Proteins of the dynamin superfamily mediate membrane fission, fusion, and restructuring events by polymerizing upon lipid bilayers and forcing regions of high curvature. The family consists of the classical dynamins and the dynamin-like proteins (DLPs). They group through common sequence organization and minimally contain an N-terminal GTPase domain, a middle domain, and a C-terminal GTPase effector domain (GED). Other than GBP1, an exception comes from the full-length crystal structure of a bacterial dynamin-like protein (BDLP) from the cyanobacterium Nostoc punctiforme. The BDLP GTPase domain dimerizes and forms the tube surface, the GTPase effector domain (GED) mediates self-assembly, and the paddle region contacts the lipids and promotes curvature.

In this work, we show the electron cryomicroscopy reconstruction of a bacterial dynamin-like protein (BDLP) helical filament decorating a lipid tube at ∼11 Å resolution. We fitted the BDLP crystal structure and produced a molecular model for the entire filament. The BDLP tube reconstruction reveals a tightly packed helical surface coating (50 nm diameter) dominated by dimeric globular densities that represent the asymmetric unit, and that connect as a zigzag with a vertical rise of 64.4 Å (correlates to Bessel order, n = −11). With the SAM label used as an anchor, the BDLP trunk was fitted into a radial spoke with the paddle oriented toward the membrane. However, the density preferentially fits the closer dimer observed in the dynamin-related human GBP1 GTPase domain with bound GDP-AlF3 (Ghosh et al., 2006). With the GTPase domain, neck and trunk docked, application of the helical parameters (rise = 3.1926 Å, rotation = 63.815°) to the asymmetric unit generates a fitted model of the complete helical filament. Nucleotide and lipid binding drive an intramolecular rearrangement in which the BDLP neck rotates ∼135° around proposed hinges 1a and 1b away from the trunk. The GTPase domain also turns ∼70° around two hinge regions so that the nucleotide binding pocket no longer points out along the trunk-neck axis but rests orthogonal to the axis. Analysis of two neighboring BDLP dimers shows that both the helical middle domain and GED run the full length of the extended molecule, making intimate contact with each other and, importantly, through a two-fold symmetry axis, making extensive contact in the neighboring molecule with their equivalent. The BDLP trunk tips just touch the outside of the inner lipid ring and form densely packed (left-handed 11-start) helices that push apart the phospholipid heads of the outer leaflet and restrict them to the spacing between each turn (∼50% of the volume in this region).

>MVNQVATDRFIQDLERVAQVRSEMSVCLNKLAETINKAELAGDSSSGKLSLERDIEDITIASKNLQQGVFRLLVLGDMKRGKSTFLNALIGENLLPSDVNPCTAVLTVLRYGPEKKVTIHFNDGKSPQQLDFQNFKYKYTIDPAEAKKLEQEKKQAFPDVDYAVVEYPLTLLQKGIEIVDSPGLNDTEARNELSLGYVNNCHAILFVMRASQPCTLGERRYLENYIKGRGLTVFFLVNAWDQVRESLIDPDDVEELQASENRLRQVFNANLAEYCTVEGQNIYDERVFELSSIQALRRRLKNPQADLDGTGFPKFMDSLNTFLTRERAIAELRQVRTLARLACNHTREAVARRIPLLEQDVNELKKRIDSVEPEFNKLTGIRDEFQKEIINTRDTQARTISESFRSYVLNLGNTFENDFLRYQPELNLFDFLSSGKREAFNAALQKAFEQYITDKSAAWTLTAEKDINAAFKELSRSASQYGASYNQITDQITEKLTGKDVKVHTTTTAEEDNSPGWAKWAMGLLSLSKGNLAGFALAGAGFDWKNILLNYFTVIGIGGIITAVTGILLGPIGFALLGLGVGFLQADQARRELVKTAKKELVKHLPQVAHEQSQVVYNAVKECFDSYEREVSKRINDDIVSRKSELDNLVKQKQTREINRESEFNRLKNLQEDVIAQLQKIEAAYSNLLAYYSHH[2x]>MQPDFDAAIVGGGPAGSAMASYLAEAGLSVAVFESEMFPRPHIGESLVPATMPVLDEIGVMPDIEAAGFPKKYGAAWTSAESRDVPHNGFTGLDHDFKAAEVMFVERDQPGVHRDYTFHVDRGKFDLILLKHAESRGAQVFQKTRVLKADFDTDPDLVTLNCRLGPRTLDFTTRMVIDASGRQTMLGNQLKVKVPDPVFNQYAIHAWFEGLDRTAMALDPAKRDYIYVHFLPLEDTWMWQIPITDTITSVGVVTQKHRFKAASADREKFFWDIVSSRKDIYDALQKAERIRPFKAEGDYSYAMRQICGDRFLLIGDAARFVDPIFSSGVSVALNSARLAAKDVIAAHRAGDFRKESFAT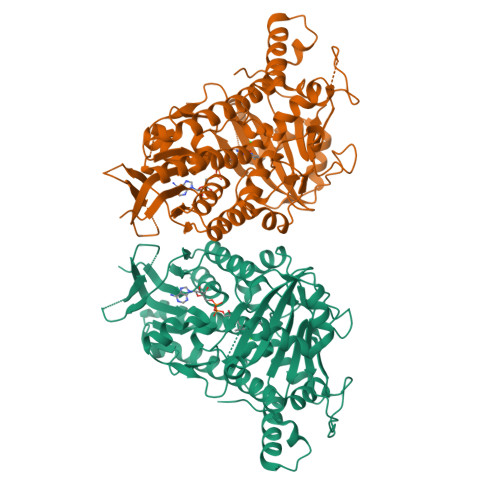YEEKLRRAVRNWYEFISVYYRLNILFTAFVQDPRYRIDVLKMLQGDFYDGEEPKALKAMRDLVTKVENDPEHLWHPYLGTLRAPSAAPTF[2x]> EEKDEEFPEQKAGEVINQPMMMAARQLHDEARKWSSKGNDIIAAAKRMALLMAEMSRLVRGGSGTKRALIQCAKDIAKASDEVTRLAKEVAKQCTDKRIRTNLLQV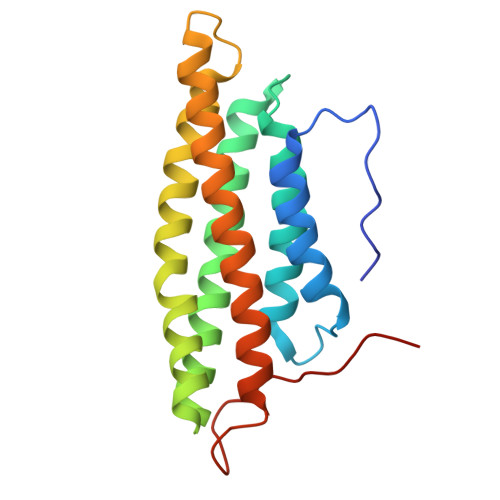CERIPTISTQLKILSTVKATMLGRTNISDEESEQATEMLVHNAQNLMQSVKETVREAEAASIKIRTDAGFTLRWVRKTPWYQ Siroheme is the modified isobacteriochlorin tetrapyrrole used by siroheme-dependent sulfite and nitrite reductases (SiR/NiRs) in catalyzing the six-electron reduction of sulfite to sulfide or nitrite to ammonia. CysG is encoded by a gene fusion between a C-terminal SUMT (CysGA) and an N-terminal bifunctional dehydrogenase/ferrochelatase (CysGB). The N-terminal enzyme module, CysGB, is a three-domain bifunctional dehydrogenase/ATP-independent class III ferrochelatase12 that performs the final two steps of siroheme biosynthesis. The C-terminal enzyme module, CysGA, is homologous to a well-studied class of SAM-dependent uro’gen III methyltransferases (SUMTs) that catalyzes the methylations to generate precorrin-210,13.

D262 comes from the CysGA module, opposing D104 but adjacent to R260/R261 and sitting above the tetrapyrrole nitrogens. Therefore, we wanted to know if D262 from CysGA was important for catalysis, so we altered it to an alanine or an asparagine (D262A or D262N). No gross structural defects were apparent. Both complemented cysG deficiency, but the altered enzymes produced the fluorescent intermediate, with defects in the dehydrogenase and chelatase activities. R261A, D262A, and D262N retain some activity for both chemistries. Given that both D262 variants retain activity, however, and its absence from Met8p, we conclude that in CysG, D262 is not strictly required. It does, however, interact with an arginine that directly binds the sirohydrochlorin, so helps form the active site to bind the tetrapyrrole in the correct orientation. P133G/H, R260A, and D262A are more sensitive to increasing cobalt concentration than D104N, R261A, or CysG.

>[2x]MDHLPIFCQLRDRDCLIVGGGDVAERKARLLLEAGARLTVNALTFIPQFTVWANEGMLTLVEGPFDETLLDSCWLAIAATDDDTVNQRVSDAAESRRIFCNVVDAPKAASFIMPSIIDRSPLMVAVSAGGTSPVLARLLREKLESLLPQHLGQVARYAGQLRARVKKQFATMGERRRFWEKFFVNDRLAQSLANADEKAVNATTERLFSEPLDHRGEVVLVGAGPGDAGLLTLKGLQQIQQADIVVYDRLVSDDIMNLVRRAADRVFVGKRAGYHCVPQEEINQILLREAQKGKRVVRLKGGDPFIFGRGGEELETLCHAGIPFSVVPGITAASGCSAYSGIPLTHRDYAQSVRLVTGHLKTGGELDWENLAAEKQTLVFYMGLNQAATIQEKLIAFGMQADMPVALVENGTSVKQRVVHGVLTQLGELAQQVESPALIIVGRVVALRDKLNWFSNH>[4x]MKARELDVPGAWEITPTIHVDSRGLFFEWLTDHGFRAFAGHSLDVRQVNCSVSSA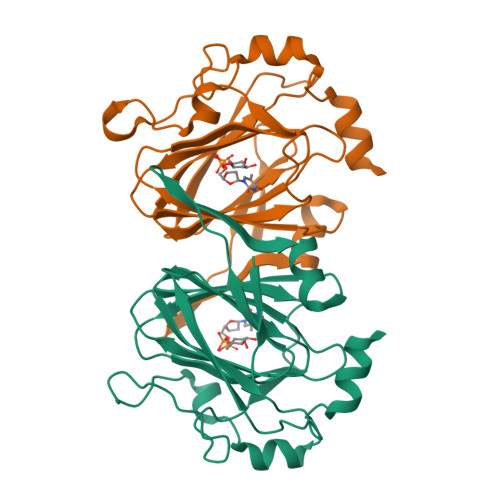GVLRGLHFAQLPPSQAKYVTCVSGSVFDVVVDIREGSPTFGRWDSVLLDDQDRRTIYVSEGLAHGFLALQDNSTVMYLCSAEYNPQREHTICATDPTLAVDWPLVDGAAPSLSDRDAAAPSFEDVRASGLLPRWEQTQRFIGEMRGT> MMAVRLTFDGQKLTWPGIGIFKATTGLPDLQWPDKQCVPDAAIPEGNYKLFIQFQ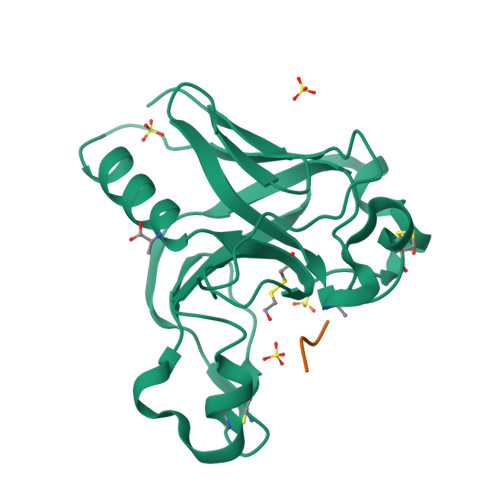GEAPIRNAADCDLGPSWGWSTIPRGQAAGTCEIYWANWGYNRIRLESADEKTRKACGGKRGGFYIHDSTKGYSHGCIEVEPVFFRILKQETEKENGEKTFTVNVKYVSGQQTNGGTKQG;> EHHHHHH> SVLLQMTQRLALSDAHFRRICQLIYQRAGIVLADHKRDMVYNRLVRRLRALGLDDFGRYLSMLEANQNSAEWQAFINALTTNLTAFFREAHHFPILAEHARRRHGEYRVWSAAASTGEEPYSIAITLADALGMAPGRWKVFASDIDTEVLEKARSGIYRLSELKTLSPQQLQR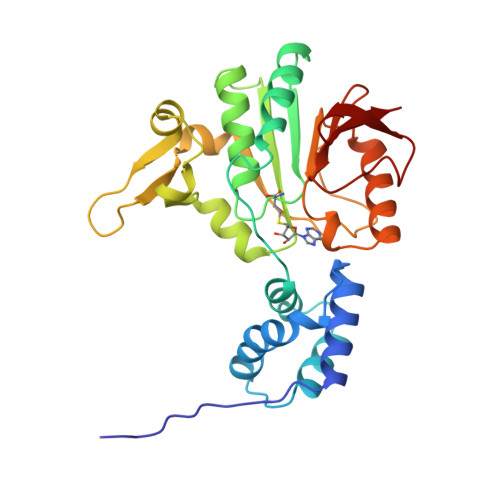YFMRGTGPHEGLVRVRQELANYVEFSSVNLLEKQYNVPGPFDAIFCRNVMIYFDKTTQEDILRRFVPLLKPDGLLFAGHSENFSNLVREFSLRGQTVYALS> GSDELYRQSLEIIS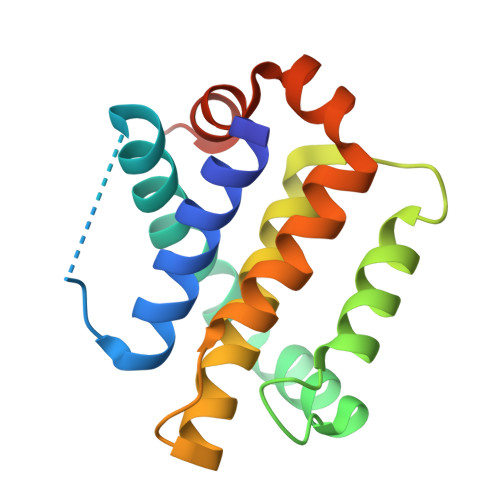RYLREQATGAKDTKPMGRSGATSRKALETLRRVGDGVQRNHETAFQGMLRKLDIKNEDDVKSLSRVMIHVFSDGVTNWGRIVTLISFGAFVAKHLKTINQESCIEPLAESITDVLVRTKRDWLVKQRGWDGFVEFFHVEDLEGG>IHIGAIFDESAKKDDEVFRTAVGDLNQNEEILQTEKITFSVTFVDGNNPFQAVQEACELMNQGILALVSSIGCTSAGSLQSLADAMHIPHLFIQRSTAGTPRSGCGLTRSNRNDDYTLSVRPPVYLHDVILRVVTEYAWQKFIIFYDSEYDIRGIQEFLDKVSQQGMDVALQKVENNINKMITTLFDTMRIEELNRYRDTLRRAILVMNPATAKSFITEVVETNLVAFDCHWIIINEEINDVDVQELVRRSIGRLTIIRQTFPVPQNISQRCFRGNHRISSTLCDPKDPFAQNMEISNLYIYDTVLLLANAFHKKLEDRKWHSMASLSCIRKNSKPWQGGRSMLETIKKGGVSGLTGELEFGENGGNPNVHFEILGTNYGEELGRGVRKLGCWNPVTGLNGSLTDKKLENNMRGVVLRVVTVLEEPFVMVSENVLGKPKKYQGFSIDVLDALSNYLGFNYEIYVAPDHKYGSPQEDGTWNGLVGELVFKRADIGISALTITPDRENVVDFTTRYMDYSVGVLLRRAEKTVDMFACLAPFDLSLWACIAG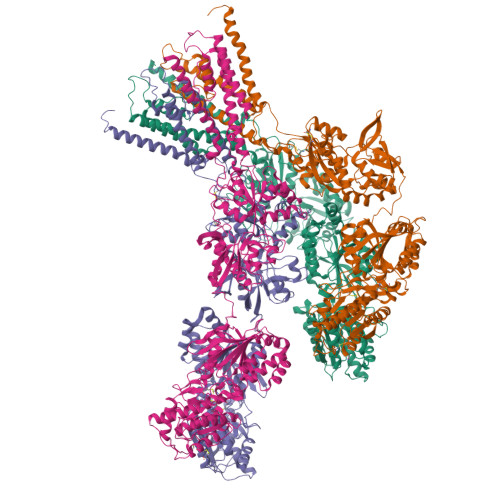TVLLVGLLVYLLNWLNPPRLQMGSMTSTTLYNSMWFVYGSFVQQGGEVPYTTLATRMMMGAWWLFALIVISSYTANLAAFLTITRIESSIQSLQDLSKQTEIPYGTVLDSAVYEHVRMKGLNPFERDSMYSQMWRMINRSNGSENNVLESQAGIQKVKYGNYAFVWDAAVLEYVAINDPDCSFYTIGNTVADRGYGIALQHGSPYRDVFSQRILELQQNGDMDILKHKWWPKNGQCDLYSSVDTKQKGGALDIKSFAGVFCILAAGIVLSCFIAMLETWWNKRKGSR[4x]>DTLDEAERQWKAEFHRWSSYMVHWKNQFDHYSKQDRCSDL[8x];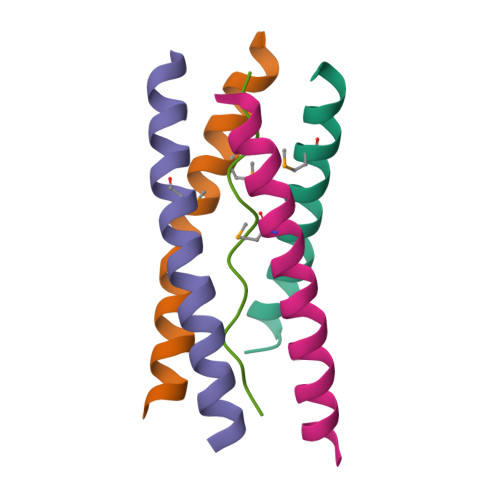>LLTPPPPPLFPPPFF[2x]>[2x]MFNRTTQLKSKHPCSVCTRRKVKCDRMIPCGNCRKRGQDSECMKSTKLITASSSKEYLPDLLLFWQNYEYWITNIGLYKTKQRDLTRTPANLDTDTEECMFWMNYLQKDQSFQLMNFAMENLGALYFGSIGDISELYLRVEQYWDRRADKNHSVDGKYWDALIWSVFTMCIYYMPVEKLAEIFSVYPLHEYLGSNKRLNWEDGMQLVMCQNFARCSLFQLKQCDFMAHPDIRLVQAYLILATTTFPYDEPLLANSLLTQCIHTFKNFHVDDFRPLLNDDPVESIAKVTLGRIFYRLCGCDYLQSGPRKPIALHTEVSSLLQHAAYLQDLPNVDVYREENSTEVLYWKIISLDRDLDQYLNKSSKPPLKTLDAIRRELDIFQYKVDSLEEDFRSNNSRFQKFIALFQISTVSWKLFKMYLIYYDTADSLLKVIHYSKVIISLIVNNFHAKSEFFNRHPMVMQTITRVVSFISFYQIFVESAAVKQLLVDLTELTANLPTIFGSKLDKLVYLTERLSKLKLLWDKVQLLDSGDSFYHPVFKILQNDIKIIELKNDEMFSLIKGLGSLVPLNKLRQESLLEEEDENNTEPSDFRTIVEEFQSEYNISDILSGSGGSGENLYFQ;> MVTSNVVLVSGEGERFTVDKKIAERSLLLKNYLNDMHDSNLQNNSDSESDSDSETNHKSKDNNNGDDDDEDDDEIVMPVPNVRSSVLQKVIEWAEHHRDSNFPDEDDDDSRKSAPVDSWDREFLKVDQEMLYEIILAANYLNIKPLLDAGCKVVAEMIRGRSPEEIRRTFNIVNDFTPEEEAAIRRENEWAEDR

The centromere is distinguished by the presence of nucleosomes containing the histone H3 variant, CENP‐A. In budding yeast, centromere establishment begins with the recognition of a specific DNA sequence by the CBF3 complex. The ~445‐kDa CBF3 complex consists of four proteins: Ndc10, Cep3, Ctf13 and Skp1 present in a 2:2:1:1 stoichiometry (Lechner & Carbon, 1991; Doheny et al, 1993; Lechner, 1994; Strunnikov et al, 1995; Stemmann & Lechner, 1996; Russell et al, 1999; Espelin et al, 1997). Previous studies have suggested that Ndc10 and Cep3 constitute the DNA‐binding activities of the complex. Both Ndc10 and Cep3 are capable of directly binding DNA (Espelin et al, 1997; Purvis & Singleton, 2008; Cho & Harrison, 2011; Perriches & Singleton, 2012); in the case of Cep3, sequence specificity for the CDEIII element is provided by zinc‐containing Gal4‐type DNA‐binding domains (Strunnikov et al, 1995; Espelin et al, 1997).

Here, we present the structure of the 220‐kDa Cep3‐Ctf13‐Skp1 (henceforth “core”) complex determined by cryo‐electron microscopy at an overall resolution of 3.6 Å. The density clearly shows that the N‐terminal F‐box forms part of a small helical domain, which is followed by seven leucine‐rich repeats (LRRs), placing Ctf13 in the sub‐class of FBXLs (F‐box proteins containing LRRs; Kipreos & Pagano, 2000). Interestingly, the Ctf13 F‐box/Skp1 interaction present in our structure is significantly different from all currently known examples, with substantially altered positioning of the helices in both the F‐box and Skp1. Our structure also highlights the function of a previously unresolved loop between residues 105 and 112 in Skp1 in forming inter‐subunit contacts. The structure provides an answer to this question. As previously described, one of the Cep3 Gal4 domains is stabilised by interactions with both Ctf13 and the F‐box binding segment of Skp1, with clear density visible at the tip of one Cep3 monomer, close to the N‐terminal of the crystal structures. The quality of the density is sufficient to visualise the Zn2Cys6 cluster, assign the correct amino acid sequence and the build the likely path of the loop connecting the domain to the rest of the Cep3 protein. By superimposing the crystal structure of the homologous Hap1 domain (King et al, 1999) bound to DNA on the Cep3 Gal4 domain, we can trace the likely path of the DNA. This modelling clearly shows a severe clash between the DNA and the LRRs of Ctf13, indicating that this domain is likely incapable of DNA binding once the complex has formed (Fig EV5A and B). It should be noted that we obtained the core structure without pre‐treatment with λ‐phosphatase; therefore, the presented structure likely represents an inactive state of the core complex.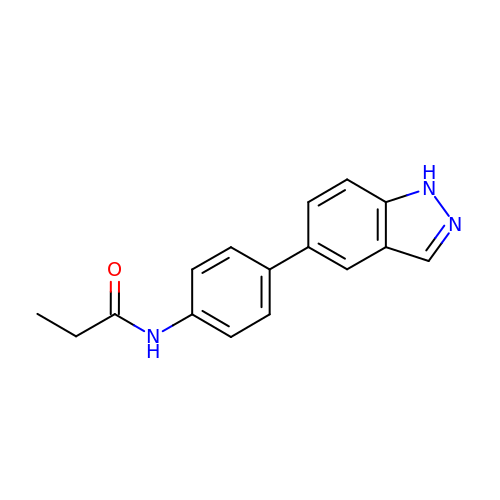N-[4-(1H-indazol-5-yl)phenyl]propanamide | C16 H15 N3 O | RLWMPXUGNDBLGJ-UHFFFAOYSA-N N-[2-({2-[(2-hydroxyethyl)amino]ethyl}amino)quinolin-5-yl]-2-[(3s,5s,7s)-tricyclo[3.3.1.1~3,7~]decan-1-yl]acetamide 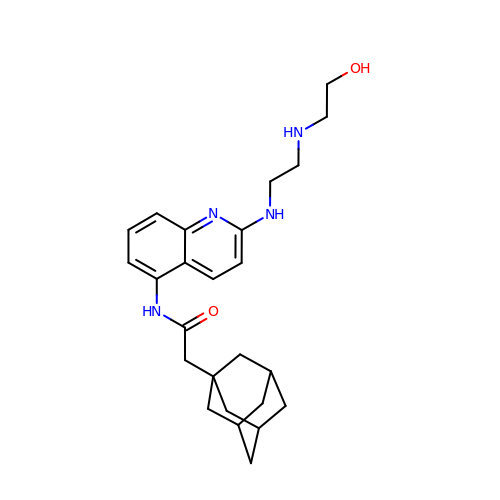| C25 H34 N4 O2 | FQMZXMVHHKXGTM-DXSJEHQWSA-N>MILKRAADVTPQKISTDKVRGVRKRVLIGLKDAPNFVIRLFTVEPGGLIDRHSHPWEHEIFVLKGKLTVLKEQGEETVEEGFFIFVEPNEIHGFRNDTDSEVEFLQLIPKEGGE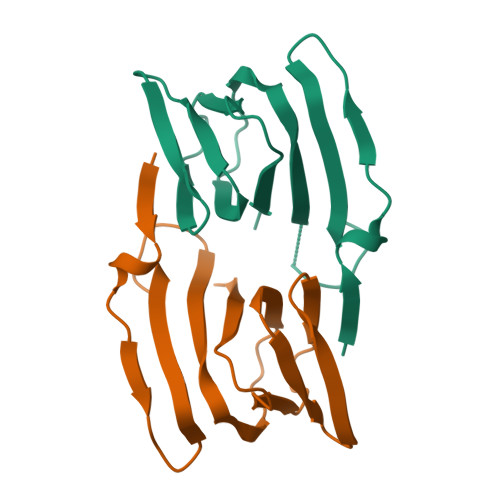[2x]Encapsulins are protein nanocompartments that house various cargo enzymes, including a family of decameric ferritin-like proteins. Cargo enzymes are directed inside the encapsulin nanocompartment by a terminal localization sequence (LS) that binds to the interior face of the encapsulin. EncFtn oxidizes iron in a similar manner to other ferritins, but due to its open structure, it must be associated with an encapsulin nanocage to act as an iron store. Together, the encapsulin EncFtn (Enc:EncFtn) complex can perform both the oxidation and storage functions of classical ferritins. Here, we investigate the structure of the Enc:EncFtn nanocompartment from the halophilic bacterium Haliangium ochraceum to gain a better understanding of the arrangement and stoichiometry of the complex.

To capture the extreme open and closed conformations of the fivefold pores, we performed symmetry expansion on the I1 particle set in Relion3.1, followed by masked 3D classification without alignment centered on the vertex. The open conformation has a fivefold pore with an aperture diameter of approximately 15 Å, while in the closed conformation the aperture is reduced to 5-Å diameter. To allow for the widening of the pore, the open pentamer protrudes from the nanocompartment by 5 Å. However, this is the first time that an open pore conformation has been observed in an encapsulin protein. Our results suggest that the flexibility of the A-domain should also be considered when engineering the pore structure for enhanced transport across the encapsulin shell. In addition, our focused refinements of the pentameric subunits allowed us to build and sequence the 117GSLGIGSLR125 peptide from the EncFtn protein. This region of the LS forms a network of hydrophobic interactions with the inner face of the P-domain of a single encapsulin monomer, with further stabilization by several water-mediated backbone contacts. Our work suggests testable hypotheses for engineering pore selectivity, through modifications to the hinge regions between the P- and A-domains, which are responsible for the opening of the pore.

>MSSEQLHEPAELLSEETKNMHRALVTLIEELEAVDWYQQRADACSEPGLHDVLIHNKNEEVEHAMMTLEWIRRRSPVFDAHMRTYLFTERPILELEEEDTGSSSSVAASPTSAPSHGSLGIGSLRQEGKED[5x];>[5x]MDLLKRHLAPIVPDAWSAIDEEAKEIFQGHLAGRKLVDFRGPFGWEYAAVNTGELRPIDDTPEDVDMKLRQVQPLAEVRVPFTLDVTELDSVARGATNPDLDDVARAAERMVEAEDSAIFHGWAQAGIKGIVDSTPHEALAVASVSDFPRAVLSAADTLRKAGVTGPYALVLGPKAYDDLFAATQDGYPVAKQVQRLVVDGPLVRANALAGALVMSMRGGDYELTVGQDLSIGYAFHDRSKVELFVAESFTFRVLEPGAAVHLRYA> AEQATKSVLFVCLGNKCRSPIAEAVFRKLVTDQNISENWVIDS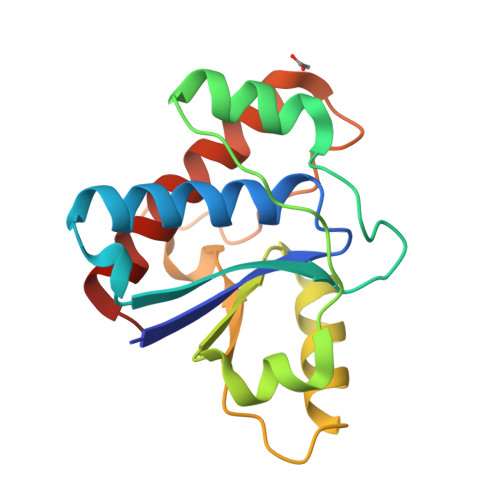GAVSDWNVGRSPDPRAVSCLRNHGIHTAHKARQITKEDFATFDYILCMDESNLRDLNRKSNQVKTCKAKIELLGSYDPQKQLIIEDPYYGNDSDFETVYQQCVRCCRAFLEKAH> MGEYIKLKVIGQD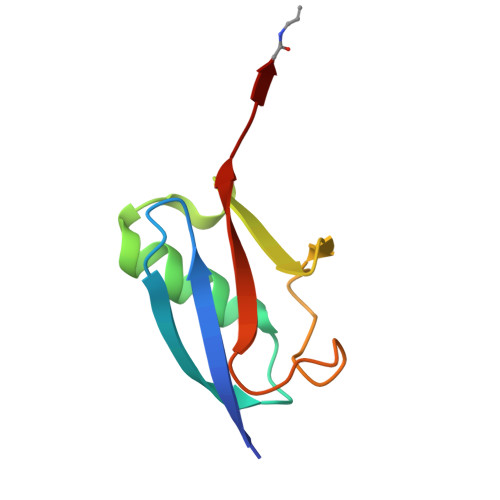SSEIHFKVKMTTHLKKLKESYCQRQGVPMNSLRFLFDGQRIADNHTPKELGMEEEDVIEVYQEQTGX>SNAMIIRPEQHWFLRLFDWHGSVLSKIIFRLLLNVLMSIIAIISYQWYEQLGIHLTVAPFSLLGIAIAIFLGFRNSASYSRFVEARNLWGTVLIAERTLVRQLRNILPAEHDAHRRIVSYLVAFSWSLKHQLRKTDPTADLRRLLPEERVTEILASSMPTNRILLLAGNEIGQLREAGKLSDITYGLMDNKLDELAHVLGGCERLAT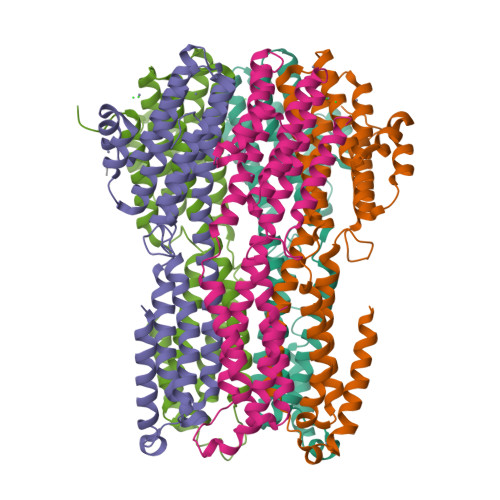TPVPFAYTLILQRTVYLFCTLLPFALVGDLHYMTPFVSVFISYTFLSWDSLAEEAEDPFGTAANDLPLNAMCNTIERNLLDMTGQHPLPE[5x]> GAASMEFPFDVDALFPERITVLDQHLRPPARRPGTTTPARVDLQQQIMTIIDELGKASAKAANLSAPITSASRMQSNRHVVYILKDSSARPAGK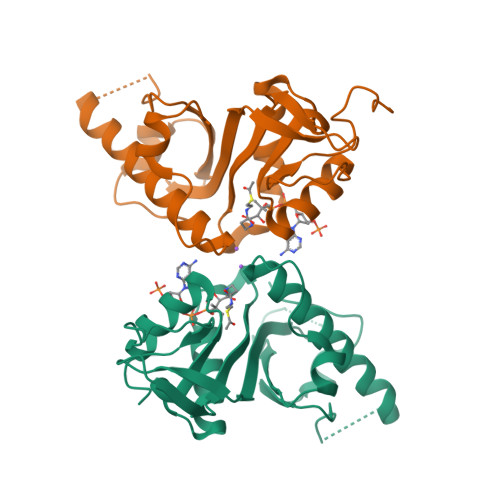GAIIGFIKVGYKKLFVLDDREAHNEVEPLCILDFYIHESVQRHGHGRELFQYMLQKERVEPHQLAIDRPSQKLLKFLNKHYNLETTVPQVNNFVIFEGFFAHQHRP;> GAASMEFPFDVDALFPERITVLDQHLRPPARRPGTTTPARVDLQQQIMTIIDELGKASAKAANLSAPITSASRMQSNRHVVYILKDSSARPAGKAAIIGFIKVGYKKLFVLDDREAHNEVEPLCILDFYIHESVQRHGHGRELFQYMLQKERVEPHQLAIDRPSQKLLKFLNKHYNLETTVPQVNNFVIFEGFFAHQHRP>[3x]MRGSHHHHHHGSMDAQSAAKCLTAVRRHSPLVHSITNNVVTNFTANGLLALGASPVMAYAKEEVADMAKIAGALVLNIGTLSKESVEAMIIAGKSANEHGVPVILDPVGAGATPFRTESARDIIREVRLAAIRGNAAEIAHTVGVTDWLIKGVDAGEGGGDIIRLAQQAAQKLNTVI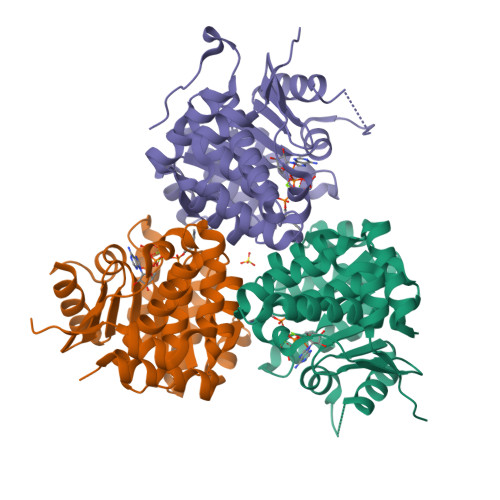AITGEVDVIADTSHVYTLHNGHKLLTKVTGAGSLLTSVVGAFCAVEENPLFAAIAAISSYGVAAQLAAQQTADKGPGSFQIELLNKLSTVTEQDVQEWATIERVTVS>[2x]MAHHHHHHMARPFLTTPPMTASNASSPATLSLARPDDWHLHLRDGDMLAAVLPHTARQFGRAIVMPNLKPPVTTTAQAQAYRERILAALPAGMTFEPLMTLYLTDNTPPDEIRRARESGFVHGVKLYPAGATTNSDHGVTDLAKCAKTLEAMQETGMPLLVHGEVTDASIDLFDREKV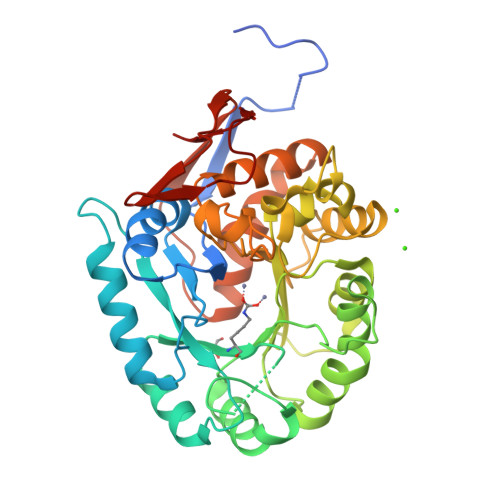FIDRVMTPLRRDFPGLKVVFEHITTKDAADYVRDADAAPGLLGATITAHHLLYNRNALFVGGIRPHYYCLPVLKRETHRVALVEAATSGNPRFFLGTDSAPHARDAKETACGCAGCYTALHALELYAEAFDTAGALDKLEGFASFFGADFYGLPRSAETVTLRREPWELPREIFAGETPVVPLRGGETIGWKLA[(2R,3S,4S,5E)-5-[[5-azanyl-2,4-bis(oxidanylidene)-1H-pyrimidin-6-yl]imino]-2,3,4-tris(oxidanyl)pentyl] 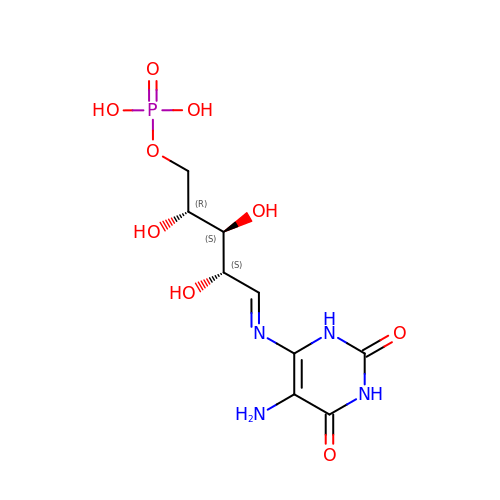dihydrogen phosphate | C9 H15 N4 O9 P | XKTZRTIKRCUGRX-ODDLNGBBSA-N>MGSSHHHHHHSSENLYFQGHMSDLPRISVAAPRLDGNERDYVLECMDTTWISSVGRFIVEFEKAFADYCGVKHAIACNNGTTALHLALVAMGIGPGDEVIVPSLTYIASANSVTYCGATPVLVDNDPRTFNLDAAKLEALITPRTKAIMPVHLYGQICDMDPILEVARRHNLLVIEDAAEAVGATYRGKKSGSLGDCATFSFFGNKIITTGEGGMITTNDDDLAAKMRLLRGQGMDPNRRYWFPIVGFNYRMTNIQAAIGLAQLERVDEHL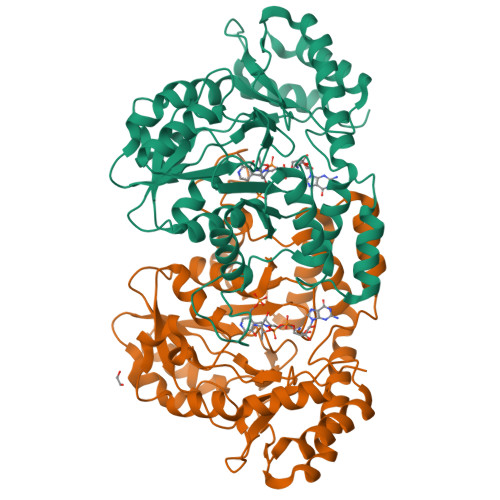AARERVVGWYEQKLARLGNRVTKPHVALTGRHVFWMYTVRLGEGLSTTRDQVIKDLDALGIESRPVFHPMHIMPPYAHLATDDLKIAEACGVDGLNLPTHAGLTEADIDRVIAALDQVLV[4x]The Rpd3L histone deacetylase (HDAC) complex is an ancient 12-subunit complex conserved in a broad range of eukaryotes that performs localized deacetylation at or near sites of recruitment by DNA-bound factors. Here we describe the cryo-EM structure of this prototypical HDAC complex that is characterized by as many as seven subunits performing scaffolding roles for the tight integration of the only catalytic subunit, Rpd3. The principal scaffolding protein, Sin3, along with Rpd3 and the histone chaperone, Ume1, are present in two copies, with each copy organized into separate lobes of an asymmetric dimeric molecular assembly. Rpd3 is the sole catalytic subunit in the Rpd3L complex.

Cryo-EM data were then acquired, processed, and the resulting map iteratively improved to 3.5 Å resolution. The cryo-EM structure of the Rpd3L complex reveals an overall architecture comprising two giant lobes attached to the stems of a two-stemmed cross-brace scaffold. Lobe I is formed largely by Rpd3, Sin3, and Sap30 and is wedged between the stems of the cross-brace. Lobe II is made up of Rxt3 and a second copy of Rpd3 and Sin3, but unlike Lobe I, engages only one of the stems. Stem I is made up of a heterodimeric, anti-parallel, two-stranded α-helical coiled-coil comprising Sds3 and Dep1. Stem II is comparatively shorter, formed by a heterodimeric, anti-parallel, four-stranded α-helical coiled-coil comprising Rxt2 and Pho23 oriented almost perpendicular to Stem I, completing the brace. Each lobe and stem together appear to form an independent structural unit. This bipartite organization takes the form of an asymmetric dimer characterized by Sin3 and Rpd3 engaging with each other extensively and almost identically in each unit of the dimer. Unexpectedly, the Rxt2 polypeptide chain snakes through many nooks and crannies in both lobes, engaging as many as six subunits and serving as a molecular glue while also stitching the two halves of the dimer together. Intriguingly, whereas the active site is readily accessible in Lobe I, the site in Lobe II is completely occluded by a segment of Rxt2. The active site tunnel is blocked near the entrance by Leu80 that mimics the conformation at both the main chain and side chain levels adopted by an Nε-acetyllysine substrate bound to an Rpd3 homologue.

>[2x]MSQVWHNSNSQSNDVATSNDATGSNERNEKEPSLQGNKPGFVQQQQRITLPSLSALSTKEEDRRDSNGQQALTSHAAHILGYPPPHSNAMPSIATDSALKQPHEYHPRPKSSSSSPSINASLMNAGPAPLPTVGAASFSLSRFDNPLPIKAPVHTEEPKSYNGLQEEEKATQRPQDCKEVPAGVQPADAPDPSSNHADANDDNNNNENSHDEDADYRPLNVKDALSYLEQVKFQFSSRPDIYNLFLDIMKDFKSQAIDTPGVIERVSTLFRGYPILIQGFNTFLPQGYRIECSSNPDDPIRVTTPMGTTTVNNNISPSGRGTTDAQELGSFPESDGNGVQQPSNVPMVPSSVYQSEQNQDQQQSLPLLATSSGLPSIQQPEMPAHRQIPQSQSLVPQEDAKKNVDVEFSQAISYVNKIKTRFADQPDIYKHFLEILQTYQREQKPINEVYAQVTHLFQNAPDLLEDFKKFLPDSSASANQQVQHAQQHAQQQHEAQMHAQAQAQAQAQAQVEQQKQQQQFLYPASGYYGHPSNRGIPQQNLPPIGSFSPPTNGSTVHEAYQDQQHMQPPHFMPLPSIVQHGPNMVHQGIANENPPLSDLRTSLTEQYAPSSIQHQQQHPQSISPIANTQYGDIPVRPEIDLDPSIVPVVPEPTEPIENNISLNEEVTFFEKAKRYIGNKHLYTEFLKILNLYSQDILDLDDLVEKVDFYLGSNKELFTWFKNFVGYQEKTKCIENIVHEKHRLDLDLCEAFGPSYKRLPKSDTFMPCSGRDDMCWEVLNDEWVGHPVWASEDSGFIAHRKNQYEETLFKIEEERHEYDFYIESNLRTIQCLETIVNKIENMTENEKANFKLPPGLGHTSMTIYKKVIRKVYDKERGFEIIDALHEHPAVTAPVVLKRLKQKDEEWRRAQREWNKVWRELEQKVFFKSLDHLGLTFKQADKKLLTTKQLISEISSIKVDQTNKKIHWLTPKPKSQLDFDFPDKNIFYDILCLADTFITHTTAYSNPDKERLKDLLKYFISLFFSISFEKIEESLYSHKQNVSESSGSDDGSSIASRKRPYQQEMSLLDILHRSRYQKLKRSNDEDGKVPQLSEPPEEEPNTIEEEELIDEEAKNPWLTGNLVEEANSQGIIQNRSIFNLFANTNIYIFFRHWTTIYERLLEIKQMNERVTKEINTRSTVTFAKDLDLLSSQLSEMGLDFVGEDAYKQVLRLSRRLINGDLEHQWFEESLRQAYNNKAFKLYTIDKVTQSLVKHAHTLMTDAKTAEIMALFVKDRNASTTSAKDQIIYRLQVRSHMSNTENMFRIEFDKRTLHVSIQYIALDDLTLKEPKADEDKWKYYVTSYALPHPTEGIPHEKLKIPFLERLIEFGQDIDGTEVDEEFSPEGISVSTLKIKIQPITYQLHIENGSYDVFTRKATNKYPTIANDNTQKGMVSQKKELISKFLDCAVGLRNNLDEAQKLSMQKKWENLKDSIAKTSAGNQGIESETEKGKITKQEQSDNLDSSTASVLPASITTVPQDDNIETTGNTESSDKGAKIQ;>[2x]MVYEATPFDPITVKPSDKRRVAYFYDADVGNYAYGAGHPMKPHRIRMAHSLIMNYGLYKKMEIYRAKPATKQEMCQFHTDEYIDFLSRVTPDNLEMFKRESVKFNVGDDCPVFDGLYEYCSISGGGSMEGAARLNRGKCDVAVNYAGGLHHAKKSEASGFCYLNDIVLGIIELLRYHPRVLYIDIDVHHGDGVEEAFYTTDRVMTCSFHKYGEFFPGTGELRDIGVGAGKNYAVNVPLRDGIDDATYRSVFEPVIKKIMEWYQPSAVVLQCGGDSLSGDRLGCFNLSMEGHANCVNYVKSFGIPMMVVGGGGYTMRNVARTWCFETGLLNNVVLDKDLPYNEYYEYYGPDYKLSVRPSNMFNVNTPEYLDKVMTNIFANLENTKYAPSVQLNHTPRDAEDLGDVEEDSAEAKDTKGGSQYARDLHVEHDNEFY;> MSQQTPQESEQTTAKEQDLDQESVLSNIDFNTDLNHNLNLSEYCISSDAGTEKMDSDEEKSLANLPELKYAPKLSSLVKQETLTESLKRPHEDEKEAIDEAKKMKVPGENEDESKEEEKSQELEEAIDSKEKSTDARDEQGDEGDNEEENNEEDNENENEHTAPPALVMPSPIEMEEQRMTALKEITDIEYKFAQLRQKLYDNQLVRLQTELQMCLEGSHPELQVYYSKIAAIRDYKLHRAYQRQKYELSCINTETIATRTFIHQDFHKKVTDLRARLLNRTTQTWYDINKERRDMDIVIPDVNYHVPIKLDNKTLSCITGYASAAQLCYPGEPVAEDLACESIEYRYRANPVDKLEVIVDRMRLNNEISDLEGLRKYFHSFPGAPELNPLRDSEINDDFHQWAQ;> MAIQKVSNKDLSRKDKRRFNIESKVNKIYQNFYSERDNQYKDRLTALQTDLTSLHQGDNGQYARQVRDLEEERDLELVRLRLFEEYRVSRSGIEFQEDIEKAKAEHEKLIKLCKERLYSSIEQKIKKLQEERLLMDVANVHSYAMNYSRPQYQKNTRSHTVSGWDSSSNEYGRDTANESATDTGAGNDRRTLRRRNASKDTRGNNNNQDESDFQTGNGSGSNGHGSRQGSQFPHFNNLTYKSGMNSDSDFLQGINEGTDLYAFLFGEKNPKDNANGNEKKKNRGAQRYSTKTAPPLQSLKPDEVTEDISLIRELTGQPPAPFRLRSD;> MARPVNTNAETESRGRPTQGGGYASNNNGSCNNNNGSNNNNNNNNNNNNNSNNSNNNNGPTSSGRTNGKQRLTAAQQQYIKNLIETHITDNHPDLRPKSHPMDFEEYTDAFLRRYKDHFQLDVPDNLTLQGYLLGSKLGAKTYSYKRNTQGQHDKRIHKRDLANVVRRHFDEHSIKETDCIPQFIYKVKNQKKKFKMEFRG;> MSVSEQDPNRAYRETQSQIYKLQETLLNSARTKNKQEEGQESNTHSFPEQYMHYQNGRNSAYDLPNVSSQSVLAFTEKHYPNKLKNLGTLYYNRFKEGSFDEDSTSYSDRHSFPYNLYDNTLPPPFLPAIGIQNINNIATLKITYEDIQASFNNIESPRKRNNEIWGCDIYSDDSDPILVLRHCGFKIGAPSGGSFHKLRRTPVNVTNQDNVTGNLPLLEGTPFDLEVELLFLPTLQKYPSVKRFDITSREWGSEATVIHDGLSYGIYSIVIKQRLDRDKPHEPNGYIKNLKWT;> MSSPANLFPGLNDITDVLEEFPLATSRYLTLLHEIDAKCVHSMPNLNERIDKFLKKDFNKDHQTQVRLLNNINKIYEELMPSLEEKMHVSSIMLDNLDRLTSRLELAYEVAIKNTEIPRGLRLGVDNHPAMHLHHELMEKIESKSNSKSSQALKSESRREAMAANRRQGEHYSASTHQQDDSKNDANYGGSRHESQDHTGNNTNSRKRANAANTNNADPETKKRKRRVATTAVSPSTISTATAVNNGRIGTSTASRGVSSVGNSNNSRISRPKTNDYGEPLYCYCNQVAYGEMVGCDGADCELEWFHLPCIGLETLPKGKWYCDDCKKKL;> MTIRSSMKNNAELESKSVLANESNIISTFTRRIIKEKSGNYQVLKRSLDGKLIYPEATGISSNRGNKLLQRSEVVTRRDLNNSKPMIEQTVFYNGSEHRLLQTNIVTDSRRKRIKFTPDINVEPVLVGDENDIDGSEKEDENITDEYYGEEDDDDLSKLVNVKEILTPILSLGDIINHKTISRTFSSPILKNLALQIILMIEKEQMSVVRYSQFLEVFLGDHPEPIYESNLNLPSYNHNLTLPEDRGASDEDDINNKNNINEVNSNSLSTEAGHINNGMEEFGEEDPFFALPRLEQSNALLSLLPSSSGSASISTLTAAEQQQLNEEIESARQLSQIALQRNKEFIRNLQKIRKSVIKANRIRGRILNWSREYLGISDDDITIPVALRVVKRGLISATTNKTTNFEEEIENTMEDGVVDDNEPDEEANRA2-[4-bromanyl-2-oxidanylidene-1'-(1~{H}-pyrazolo[4,3-b]pyridin-5-ylcarbonyl)spiro[indole-3,4'-piperidine]-1-yl]-~{N}-[2,2,2-tris(fluoranyl)ethyl]ethanamide | 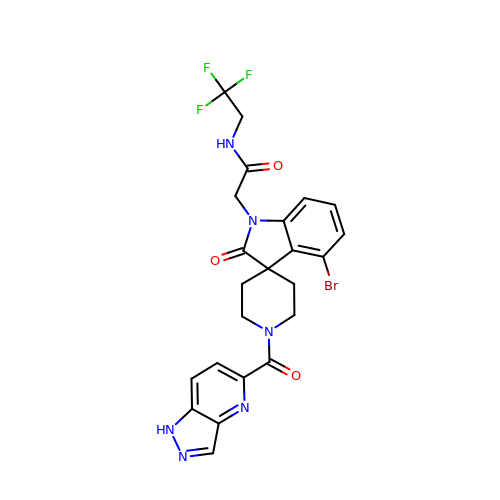C23 H20 Br F3 N6 O3 | UXEXYURPAPXPSR-UHFFFAOYSA-N> MEAAHSKSTEECLAYFGVSETTGLTPDQVKRHLEKYGHNELPAEEGKSLWELVIEQFEDLLVRILLLAACISFVLAWFEEGEETITAFVEPFVILLILIANAIVGVWQERNAENAIEALKEYEPEMGKVYRADRKSVQRIKARDIVPGDIVEVAVGDKVPADIRILSIKSTTLRVDQSILTGESVSVIKHTEPVPDPRAVNQDKKNMLFSGTNIAAGKALGIVATTGVSTEIGKIRDQMAATEQDKTPLQQKLDEFGEQLSKVISLICVAVWLINIGHFNDPVHGGSWIRGAIYYFKI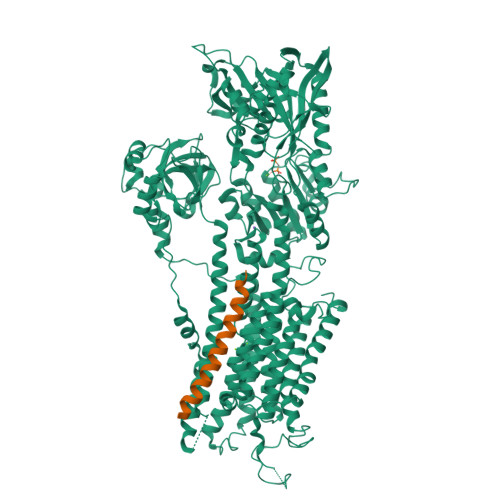AVALAVAAIPEGLPAVITTCLALGTRRMAKKNAIVRSLPSVETLGCTSVICSDKTGTLTTNQMSVCKMFIIDKVDGDFCSLNEFSITGSTYAPEGEVLKNDKPIRSGQFDGLVELATICALCNDSSLDFNETKGVYEKVGEATETALTTLVEKMNVFNTEVRNLSKVERANACNSVIRQLMKKEFTLEFSRDRKSMSVYCSPAKSSRAAVGNKMFVKGAPEGVIDRCNYVRVGTTRVPMTGPVKEKILSVIKEWGTGRDTLRCLALATRDTPPKREEMVLDDSSRFMEYETDLTFVGVVGMLDPPRKEVMGSIQLCRDAGIRVIMITGDNKGTAIAICRRIGIFGENEEVADRAYTGREFDDLPLAEQREACRRACCFARVEPSHKSKIVEYLQSYDEITAMTGDGVNDAPALKKAEIGIAMGSGTAVAKTASEMVLADDNFSTIVAAVEEGRAIYNNMKQFIRYLISSNVGEVVCIFLTAALGLPEALIPVQLLWVNLVTDGLPATALGFNPPDLDIMDRPPRSPKEPLISGWLFFRYMAIGGYVGAATVGAAAWWFMYAEDGPGVTYHQLTHFMQCTEDHPHFEGLDCEIFEAPEPMTMALSVLVTIEMCNALNSLSENQSLMRMPPWVNIWLLGSICLSMSLHFLILYVDPLPMIFKLKALDLTQWLMVLKISLPVIGLDEILKFIARNYLEG;> MERSTRELCLNFTVVLITVILIWLLVRSYQY>MTPDVLKNIADTLEARREAAPQSSYVASLFHKGEDAILKKVAEEAAETLMASKDKDKLHLVREVADLWFHTMVLLTYHGLRPEDVVMELHRREGISGL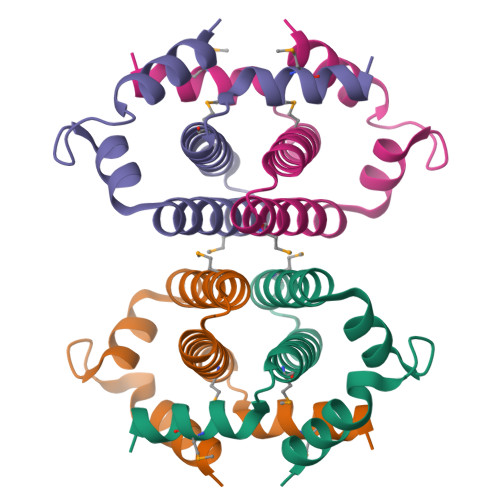DEKASRKPTALEHHHHHH[12x]> MGSSHHHHHHSSGLVPRGSHMQEQTAKEDVADSATSVGAIVSIEKAEKNFVITYASGKKAQISILNDHLFRYHLDPTGKFEEYPTPNDPKHVAKITAKTMADYGTQAFEQTNVTDSGNQFILENNGLKIIFEKESALMKVLDKKKNQVILEETAPLSFKNDKATQTLKQSSQENYFGGGTQNGRFTHKGTAIQIVNTNNWVDGGVASPNPFYWSTAGYGVVRNTWKPGNYDFGSHDPQTTTTTHEGTDFDAFYFFNDSSAGILKDYYELTGKPALMPEYGFYEAHLNAYNRDYWVKVAEGTAGAVKFEDGNFYKEYQPGDLGNLNGTLESLNGEKENYQFSARAVIDRYKKNDMPLGWFLPNDGYGAGYGQTDSLDGDVQNLKEFTDYAQANGVEVGLWTQSNLHPADPKNPKKGERDIAKEVSVAGVKALKTDVAWVGYGYSFGLNGVEDAANVFVKETDGAVRPMIVSLDGWAGTQRHAGIWTGDQTGGQWEYIRFHIPTYIGTSLSGQPNVGSDMDGIFGGKNKEVNIRDFQWKTFTPVQLNMDGWGSNPKTPFAFDQEATDLNRAYLKLKSMMMPYNYSIAKESVDGLPMVRAMALEFPNEGTAYTKDSQYQYMWGPNLLVAPIYNGNQDEAGNSIRDGIYLPDEKQVWVDLFTGEKYQGGRVLNGVKTPLWKVPVFVKDGSIIPMTNPNNNPKEIQRDQRSFLIYPNGATSFNMYEDDGISTSYEAGQSATTKINSQGPKSNEKGDLTVTIEPTKGSYKDFVD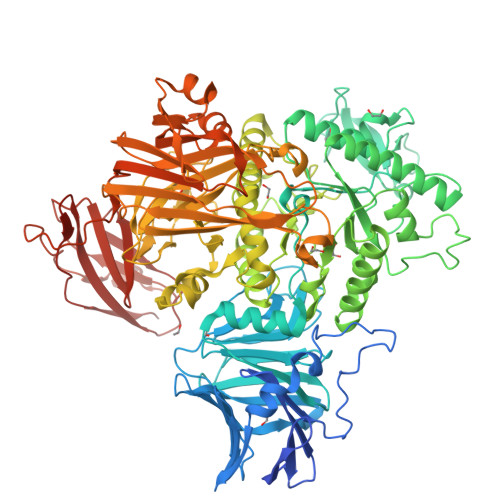ERSTTLDLLASEAPESVTAMVGGTEVTLKQAANKEEFLAGTNLYYFDKEFQVNQYLSEASGEKLNQSALSVKLAKQSVTAKDVQITVKGFINKGTVDGGNTTVDDQLTIPANIAINEEKTTPSSLTLQWDQVTEATSYEVERDGTVFGNIQTNTATFDGFSFLSEHTFRVRAVGKNGVSEWSEPIKGKTQDDPYK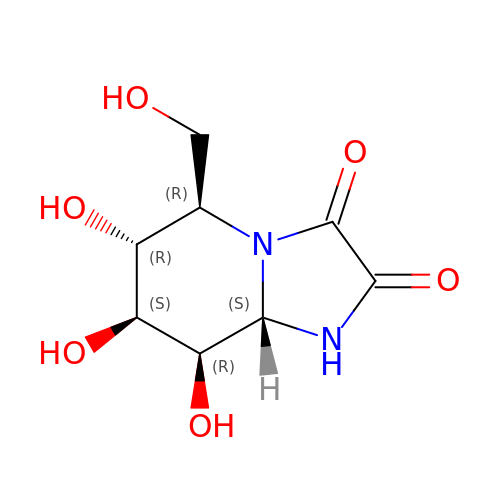KIFUNENSINE | C8 H12 N2 O6 | OIURYJWYVIAOCW-PQMKYFCFSA-N> MHSPNPLLVAPTPPALQKLLESFKIQYLQFLAYTKTPQYKASLQELLGQEKEKNAQLL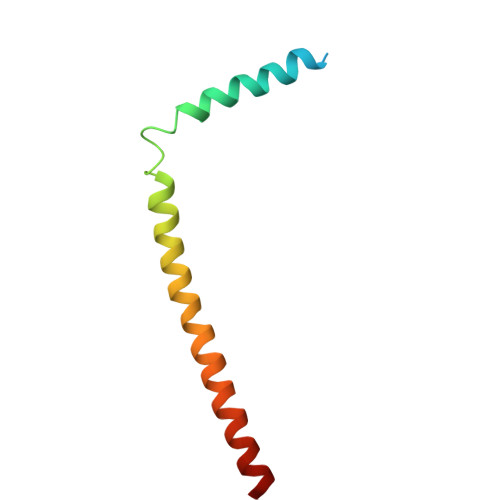GAAQQLLSHCQAQKEEIRRLFQQK> KPKGHPHMNSIRIDGDITLGGLFPVHGRGSEGKPCGELKKEKGIHRLEAMLFALDRINNDPDLLPNITLGARILDTCSRDTHALEQSLTFVQALIEKDGTEVRCGSGGPPIITKPERVVGVIGASGSSVSIMVANILRLFKIPQISYASTAPDLSDNSRYDFFSRVVPSDTYQAQAMVDIVRALKWNYVSTVASEGSYGESGVEAFIQKSREDGGVCIAQSVKIPREPKAGEFDKIIRRLLETSNARAVIIFANEDDIRRVLEAARRANQTGHFFWMGSDSWGSKIAPVLHLEEVAEGAVTILPKRMSVRGFDRYFSSRTLDNNRRNIWFAEFWEDNFHCKLSRHALKKGSHVKKCTNRERIGQDSAYEQEGKVQFVIDAVYAMGHALHAMHRDLCPGRVGLCPRMDPVDGTQLLKYIRNVNFSGIAGNPVTFNENGDAPGRYDIYQYQLRNDSAEYKVIGSWTDHLHLRIERMHWPGSGQQLPRSICSLPCQPGERKKTVKGMPCCWHCEPCTGYQYQVDRYTCKTCPYDMRPTENRTGCRPIPIIKLEWGSPWAVLPLFLAVVGIAATLFVVITFVRYNDTPIVKASGRELSYVLLAGIFLCYATTFLMIAEPDLGTCSLRRIFLGLGMSISYAALLTKTNRIYRIFEQGKRSVSAPRFISPASQLAITFSLISLQLLGICVWFVVDPSHSVVDFQDQRTLDPRFARGVLKCDISDLSLICLLGYSMLLMVTCTVYAIKTRGVPETFNEAKPIGFTMYTTCIVWLAFIPIFFGTSQSADKLYIQTTTLTVSVSLSASVSLGMLYMPKVYIILFHPEQNVPKRKRSLKAVVTAATMSNKFTQKGNFRPNGEAKSELCENLEAPALATKQTYVTYTNHAI;> EGPAKKVLTLEGDLVLGGLFPVHQKGGPAEDCGPVNEHRGIQRLEAMLFALDRINRDPHLLPGVRLGAHILDSCSKDTHALEQALDFVRASLSRGADGSRHICPDGSYATHGDAPTAITGVIGGSYSDVSIQVANLLRLFQIPQISYASTSAKLSDKSRYDYFARTVPPDFFQAKAMAEILRFFNWTYVSTVASEGDYGETGIEAFELEARARNICVATSEKVGRAMSRAAFEGVVRALLQKPSARVAVLFTRSEDARELLAASQRLNASFTWVASDGWGALESVVAGSEGAAEGAITIELASYPISDFASYFQSLDPWNNSRNPWFREFWEQRFRCSFRQRDCAAHSLRAVPFEQESKIMFVVNAVYAMAHALHNMHRALCPNTTRLCDAMRPVNGRRLYKDFVLNVKFDAPFRPADTHNEVRFDRFGDGIGRYNIFTYLRAGSGRYRYQKVGYWAEGLTLDTSLIPWASPSAGPLPASRCSEPCLQNEVKSVQPGEVCCWLCIPCQPYEYRLDEFTCADCGLGYWPNASLTGCFELPQEYIRWGDAWAVGPVTIACLGALATLFVLGVFVRHNATPVVKASGRELCYILLGGVFLCYCMTFIFIAKPSTAVCTLRRLGLGTAFSVCYSALLTKTNRIARIFGGAREGAQRPRFISPASQVAICLALI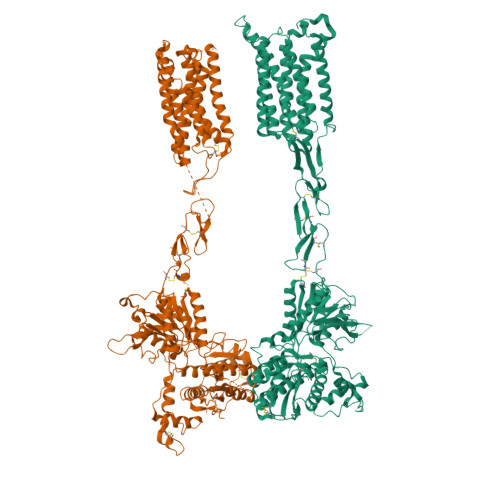SGQLLIVVAWLVVEAPGTGKETAPERREVVTLRCNHRDASMLGSLAYNVLLIALCTLYAFKTRKCPENFNEAKFIGFTMYTTCIIWLAFLPIFYVTSSDYRVQTTTMCVSVSLSGSVVLGCLFAPKLHIILFQPQKNVVSHRAPTSRFGSAAARASSSLGQGSGSQFVPTVCNGREVVDSTTSSL> MDSITKLFGDLCESHMVGFPWRTALNSRKHSKNRTKQTLKKLAYDTLFVHLFQDEARKLQPNCTRLPVKNKIIMLSFNLRICGMSSEADRLEELVEYLEQSNGIQISDLHAVLELLVELSGTGPPQLLPPKRDYFKNNKYVGRNVKYQGYDYYDVQVFEADLGTTVAYQELEISTTIQRTLQIMEAAPGTGLPALSFFSQNDLSTDKFEKETRGSLFGALVHSRTNDMDIKLDMPPVPENADLSGLAIKVPQSIDQSEDEGFQSASNMTPDSQSEPSMTPDIDVWEAVLTYGPSKRRCWERIGCPPGKREEPYVTEAGREAFDKLYKLHEGGLQILSATTLQPQLVLLEETDLVKAVLNVLIGVVSSTFSYNQALQSFAVKQGVYISGTSPDNVSSLLTQVAEYGTYYTRLSHFSLLTVLDSSHSNGLVFQAFTSGLRKYLQYYRACVLSTPASLTLLTISFLFRKLGRQLRYLAELCCIGTLVTSATRGISTAFPTGVKLLSYLYKEALENSSNENYPVLLSLLKTSCEPYTRFIYDWVYSGVFRDVCGEFMIQVNEDYLGFRDKRYWTHGYVLISKEVEDCVPVFLKHVANEIYICGKTINLLKLCCPKHYICWSDIPVPRISVTFSLEELKEMEKDCAVYVARMERIARHSCISKEQKALQTEIARQELIIQARETTEKVFETFKDRKLAEKLSLDTKKRELFQKLKDQYEKEQERRLTTKQEEADDDFSYAREIRDREKRLKALEEELELKTRQELIEHYSRLSEEATRKEQRALWKLQRHKLETIRLKFFLEEQKRMQDLVANFPVDICEENLGVLPDGEISHQTDNTNDAGLGNIENEKSVPEQHALHNNNDEVYTAQNCISKSESLCVDVTLPTENVHSQTSNASVLGVPSFDSNLCTPDVDIIDFLPTLPSENQEVAVVQSLVDDALISIGSDLNTDTKDKESLCALKSDLQESSTGSEYDFKTILKPIACTQVSQGHIKIGEYSSNVQPARPRWSTHGHSSDSNIKIGNYVSDINVHQPKHSQHGHSSDSNINISDHMSDVEPRLPRLNLHGHISTGHIKVGEYASDVEPSTPRHSVHGHASQGNIKIGENVSDVKLSRPRWNIHGHVSDANIKIGENTSEIAPLRPRWNIHGHASQSHIKIGELVSDIEPSQPRRTPFGHPSQSSIPIGDQPVEKYAQKSESEVHSSNSTIQHLLYSNIPDKNKDTGGTLTDSPVPVPDQGNSNDDTEKRSSTLEQRVQAADSVCDGEASPN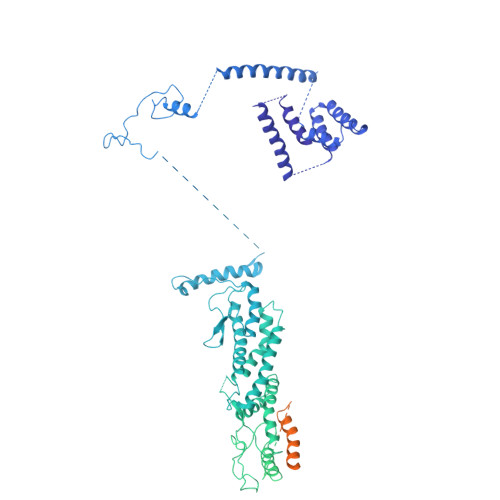TAQSLPCMSDTLDFGTNGEENVGNDDHTWEKQQEYLKGLAEKYCLEKYQDSYELMSHPPVLHLYSNVMPNRFSFPTDSDIKSATDETTVQLIELLSLPVLMKYSVTAPMVSHVYLVNKAIVDYYFVELKMERHFEAMRHFLLMEDGEFAQSLSDMLFEKLGSGQTPSELLNPLVLNSILNKALQYSLHGDSSLASNLTFALKYLPEVFTPTAPDALSCLELKYKVDWPLNIVITDTCMNKYSRIFSFLLQLKHMVWTLRDVWFHLKRTALVNQASNSVQYRQLQLYRHEMQHFVKVIQGYIANQILHVTWCEFRNKLSAVSNLEEIYKTHADYLNKALFRGLLTEKAAPLMNIIHSIFSLILKFRLQLISQSWICDTGKQMAVHPNFGLMQQSYNTFKYYSDFLFEVVSKLVNRGYQPHLEDFLLRINFNSYYKQS>[4x]HHHHHHFNLPPGNYKKPVLLYCSNGGHFLRILPDGTVDGTRDRS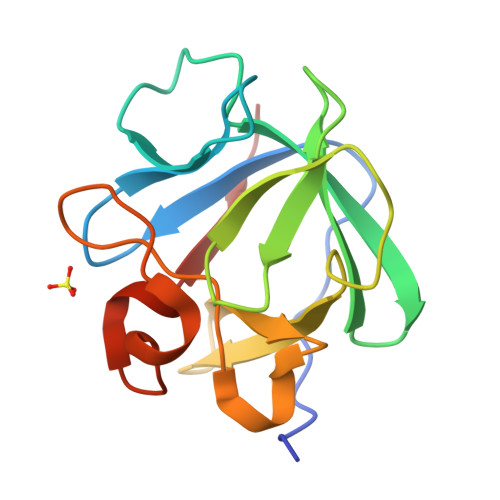DQHIQLQLSAESVGEVYIKSTETGQYLAMDTDGLLYGSQTPNEEILFLERLEENHYNTYISKKHAEKNWFVGLKKNGSVKRGPRTHYGQKAILFLPLPVSSD>HHH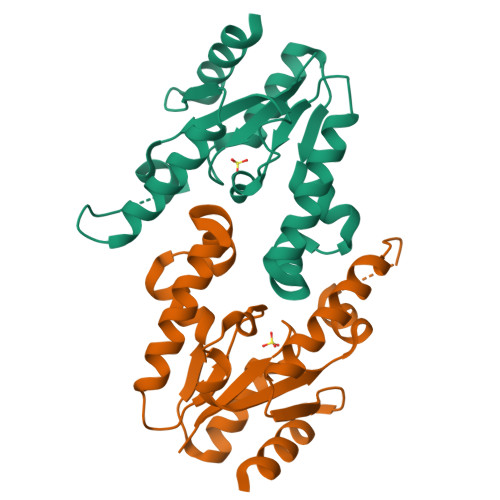HHHMQHLVLIGFMGSGKSSLAQELGLALKLEVLDTDMIISERVGLSVREIFEELGEDNFRMFEKNLIDELKTLKTPHVISTGGGIVMHENLKGLGTTFYLKMDFETLIKRLNQKEREKRPLLNNLTQAKELFEKRQALYEKNASFIIDARGGLNNSLKQVLQFIA[2x]HvExoI releases a single Glc from non-reducing termini of oligo- and polymeric β-d-glucosides to support seed germination and plant development. HvExoI folds in an (α/β)8 barrel (domain 1) and an (α/β)6 sandwich (domain 2) that at their interface cradle a 13 Å-deep pocket- or crater-shaped active site. A vital conclusion drawn from the structural studies with the native β-d-glucan glucohydrolase, isoenzyme ExoI (HvExoI) isolated from barley seedlings, was that the glucose (Glc) product released from β-d-glucoside substrates remains entrapped in the enzyme active site until an incoming substrate binds, presumably lowering the energy barrier to facilitate Glc displacement. We discover that through chemical signalling, the incoming substrate evokes the formation of an autonomous and transient lateral cavity that serves as a conduit for the Glc product displacement from the active site.

We use the high-resolution X-ray crystallography supported with enzyme kinetics, mass spectrometry, nuclear magnetic resonance (NMR) spectroscopy, multi-scale molecular modelling employing docking, Molecular dynamics (MD) simulations, Genetic Algorithms with Unrestricted Descriptors for Intuitive Molecular Modelling (GaudiMM)20 and Protein Energy Landscape Exploration (PELE)21 calculations, to reveal the Glc product displacement route, and to extract how each hydrolytic event including Glc release is precisely coordinated with the incoming substrate association and hydrolysis. This leads us to generate a variant enzyme and probe it for Glc entrapment and the S-glycoside analogue binding. Strikingly, when the toll-like barrier is disrupted in the R158A/E161A variant, Glc no longer binds in the active site, which underlines the vital role of the barrier in Glc entrapment.

> HHAADYVLYKDATKPVEDRVADLLGRMTLAEKIGQMTQIERLVATPDVLRDNFIGSLLSGGGSVPRKGATAKEWQDMVDGFQKACMSTRLGIPMIYGIDAVHGQNNVYGATIFPHNVGLGATRDPYLVKRIGEATALEVRATGIQYAFAPCIAVCRDPRWGACYASYSEDRRIVQSMTELIPGLQGDVPKDFTSGMPFVAGKNKVAACAKHFVGDGGTVDGINENNTIINREGLMNIHMPAYKNAMDKGVSTVMISYSSWNGVKMHANQDLVTGYLKDTLKFKGFVISDWEGIDRITTPAGSDYSYSVKASILAGLDMIMVPNKYQQFISILTGHVNGGVIPMSRIDDAVTRILRVKFTMGLFENPYADPAMAEQLGKQEHRDLAREAARKSLVLLKNGKTSTDAPLLPLPKKAPKILVAGSHADNLGYQCGGWTIEWQGDTGRTTVGTTILEAVKAAVDPSTVVVFAENPDAEFVKSGGFSYAIVAVGEHPYTETKGDNLNLTIPEPGLSTVQAVCGGVRCATVLISGRPVVVQPLLAASDALVAAWLPGSEGQGVTDALFGDFGFTGRLPRTWFKSVDQLPMNVGDAHYDPLFRLGYGLTTNATKKY>[2x]MRLFLSLPVLVVVLSIVLEGPAPAQGTPDVSSALDKLKEFGNTLEDKARELISRIKQSELSAKMREWFSETFQKVKEKLKIDS

Apolipoprotein C-1 (APOC1) is a 57 amino acid polypeptide of Mr = 6.6 kDa that is synthesized predominantly in the liver of mammals. In humans, the plasma concentration is about 6 mg/dl. This small protein is remarkable for being the most positively charged protein in the human body, with a lysine content of 17%. The protein has a high affinity for lipid surfaces, particularly chylomicrons, and both HDL and VLDL particles. APOC1 had long been known to be a crucial player in the transfer of lipids between particles and the general clearance of lipids, but its mechanism and the manner by which it bound to lipoprotein particles was poorly understood. It was then discovered that APOC1 is a potent inhibitor of cholesteryl ester transferase protein (CETP), which is the crucial enzyme in the transfer of cholesterol between lipid surfaces (tissues) and lipid particles.

The dimer from crystal Monocl-1, once known, was simply placed in the unit cell of Monocl-2 with the same coordinates; the two helices in the dimer were rigid body-refined and then subjected to restrained refinement. Although the movement of the two monomers within the dimer toward one another is slight, it significantly increases the interactions between them. The buried surface area is enlarged an additional 7% to 4,050 Å2 and becomes 22% of the entire surface area (19,021 Å2) of the entire dimer. Monocl-2 represents the dimer exhibiting the greatest degree of compression of the constituent monomer helices. As in Monocl-1, the hydrophobic stack interaction at one end of the dimer is fully maintained, but the opposite end of the dimer shows the two monomers pressed more closely together. In Monocl-2, the hydrophilic interactions appear a bit more certain and involve Arg39A-Ser27B, Ser43A/Glu47A-Arg 23B, and Lys 50-Glu19B/Asn16B/Asp20B. In the less hydrated (34% solvent) Monocl-1 crystals, and the even less hydrated (25% solvent) Monocl-2 crystals, dimers are so closely packed, molecule A against B of translationally related dimers, that the sheet or band is extremely dense. Although the band seen in Monocl-2 likely represents the compression limit (the monomers can get no closer to one another), it is not certain that the bands found in Monocl-3 are necessarily the limit of maximum expansion.>[2x]MT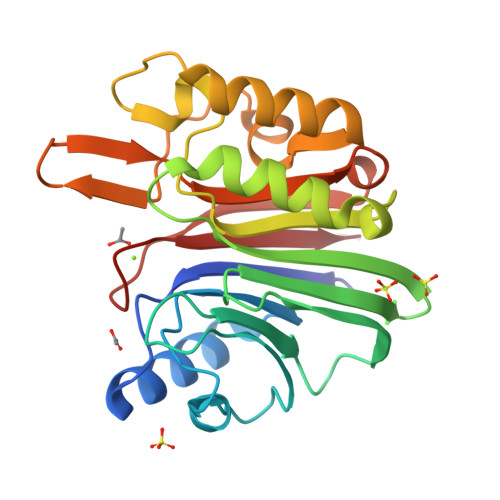GSNSHITILTLNINGLNSAIKRHRLASWIKSQDPSVCCIQETHLTCRDTHRLKIKGWRKIYQANGKQKKAGVAILVSDKTDFKPTKIKRDKEGHYIMVKGSIQQEELTILNIYAPNTGAPRFIKQVLSDLQRDLDSHTLIMGDFNTPLSTLDRSTRQKVNKDTQELNSALHQADLIDIYRTLHPKSTEYTFFSAPHHTYSKIDHIVGSKALLSKCKRTEIITNYLSDHSAIKLELR> FYSVEVADSTFTVLKRYQQLKPIGSGAQGIVCAAFDTVLGINVAVKKLSRPFQNQTHAKRAYRELVLLKCVNHKNIISLLNVFTPQKTLEEFQDVYLVMELMDANLCQVIHMELDHERMSYLLYQMLCGIKHLHSAGIIHRDLKPSNIVVKSDCTLKILDFGLARTACTNFMMTPYVVTRYYRAPEVILGMGYAANVDIWSVGCIMGELVKGCVIFQGTDHIDQWNKVIEQLGTPSAEFMAALQPTVRNYVENRPKYPGIKFEELFPDWIFPSESERDKIKTSQARDLLSKMLVIDPD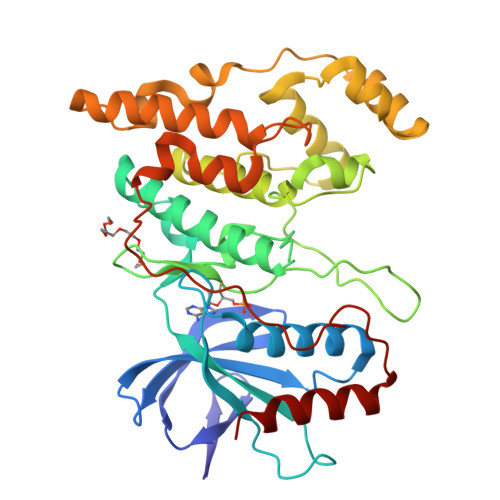KRISVDEALRHPYITVWYDPAEAEAPPPQIYDAQLEEREHAIEEWKELIYKEVMDWE>MNSNVENLPPHIIRLVYKEVTTLTADPPDGIKVFPNEEDLTDLQVTIEGPEGTPYAGGLFRMKLLLGKDFPASPPKGYFLTKIFHPNVGANGEICVNVLKRDWTAELGIRHVLLTIKCLLIHPNPESALNEEAGRLLLEN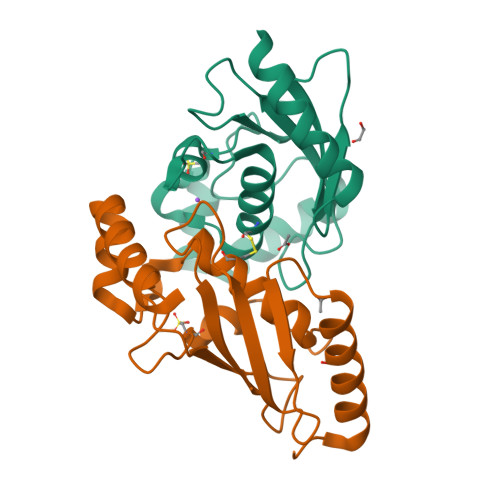YEEYAARARLLTEIHG[2x]> MENTENSVDSKSIKNLEPKII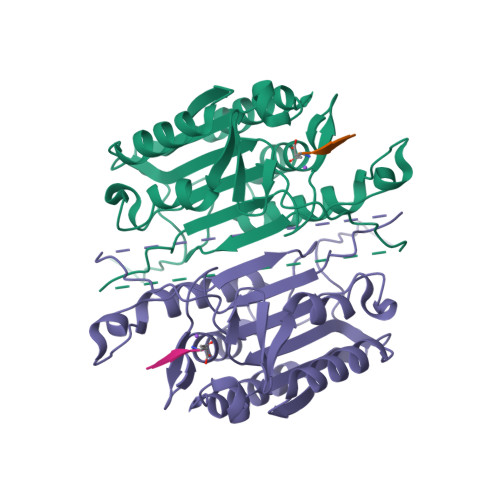HGSESMDSGISLDNSYKMDYPEMGLCIIINNKNFHKSTGMTSRSGTDVDAANLRETFRNLKYEVRNKNDLTREEIVELMRDVSKEDHSKRSSFVCVLLSHGEEGIIFGTNGPVDLKKITNFFRGDRCRSLTGKPKLFIIQACRGTELDCGIETDSGVDDDMACHKIPVEADFLYAYSTAPGYYSWRNSKDGSWFIQSLCAMLKQYADKLEFMHILTRVNRKVATEFESFSFDATFHAKKQIPCIASMLTKELYFYHL The dihydrouridine biosynthetic reaction is catalyzed by a large family of flavoenzymes, the dihydrouridine synthases (Dus). Dus2 is the eukaryotic enzyme responsible for the synthesis of D20 in tRNAs and is involved in some human cancers and in the detoxification of β-amyloid peptides in Alzheimer’s disease. Overall, the structural analyses of all these structures allow for the definition of a canonical Dus fold, which consists of: (i) a TIM-barrel domain on the N-terminal side carrying the active site with the FMN located in the center of the barrel; (ii) a helical domain (HD) formed by 4 helices in a bundle lying on the C-terminal side; and (iii) a linker, which connects these two domains. In contrast, hDus2 was shown to carry an additional domain after the HD, namely a double-strand binding domain (dsRBD) cooperating with the TIM-barrel for tRNA recognition and binding.

The other domain acquired by more evolved Dus2 is the dsRBD. By reanalyzing the sequences of eukaryotic Dus2, we found out that the dsRBD does not seem to be restricted to animals but is also present in Choanoflagellates and in Filasterea, all of which are part of the Filozoa clade. To determine if the dsRBDs of animals at the bottom of the evolutionary tree retain the same double-stranded RNA recognition mechanism compared to the dsRBD of hDus2, we crystallized the dsRBD of Dus2 from A. queenslandica, Monosiga brevicolis, and F. alba. Unfortunately, only A. quenslandica dsRBD led to diffracting crystals that allowed structural resolution. Interestingly, the validity of these models is supported by the superposition of the crystallographic structure of A. quenslandica dsRBD, which we solved at 1.68 angstroms in this study, with the dsRBD coming from the model (RMSD = 0.426 over 78 atoms). It is equally amazing to see that even the orientations of the side chains observed in the crystal structure are globally preserved in the model. A focus on specifically the dsRBD revealed that the overall structure is conserved among all the models. We showed that recognition of dsRNA is essentially achieved via three major canonical regions, namely helix-α1, helix-α2, and the C-terminal part of the β1–β2 loop of the dsRBD. These regions are all present in all dsRBDs analyzed here. In contrast, only one of these positively charged residues is observed in F. alba (R400) and A. queenslandica (K381).

>MKSKMDPEVTEDGTLELFIRYESKDYINVPTPKVYLNDWTTRERLPIKYNTVQRSKDQLFKSTLTIKDTCYSSSLWAKSKRNAEQSAAMVALEIIGIKTPQSTASNSHHHHHH[2x]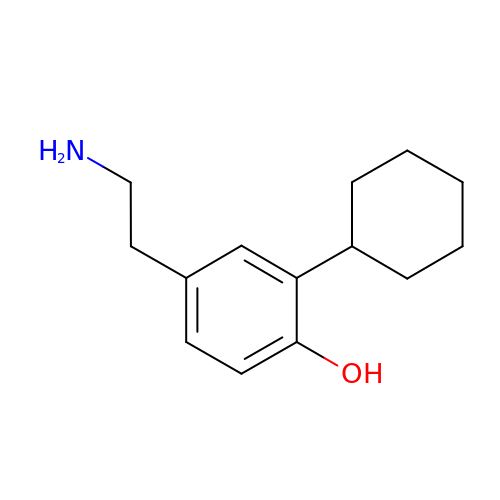4-(2-aminoethyl)-2-cyclohexylphenol | C14 H21 N O | DOCCSEDGBYCYLS-UHFFFAOYSA-N>[4x]VTAFLGERVTLTSYWRRVSLGPEIEVSWFKLGPGEEQVLIGRMHHDVIFIEWPFRGFFDIHRSANTFFLVVTAANISHDGNYLCRMKLGETEVTKQEHLSVVKPLTLSVHSERSQFPDFSVLTVTCTVNAFPHPHVQWLMPEGVEPAPSAANGGVMKEKDGSLSVAVDLSLPKPWHLPVTCVGKNDKEEAHGVYVSGYLSQKHHHHHH;>GSHMKEVS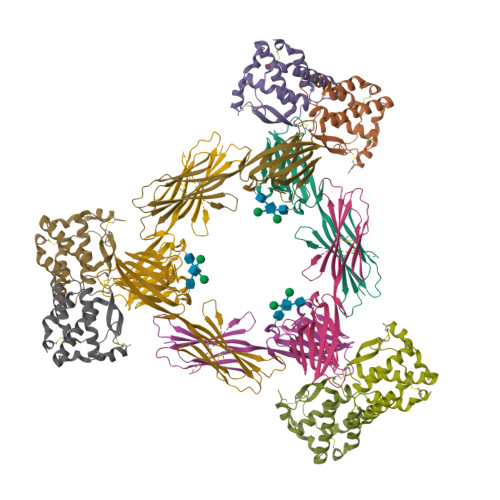EHCSHMIGNGHLKVLQQLIDSQMETSCQIAFEFVDQEQLDDPVCYLKKAFFLVQDIIDETMRFKDNTPNANATERLQELSNNLNSCFTKDYEEQNKACVRTFHETPLQLLEKIKNFFNETKNLLEKDWNIFTKNCNNSFAKCSSR[4x]>[2x]APTENSTGVQDCYRGDGQSYRGTLSTTITGRTCQSWSSMTPHWHRRIPLYYPN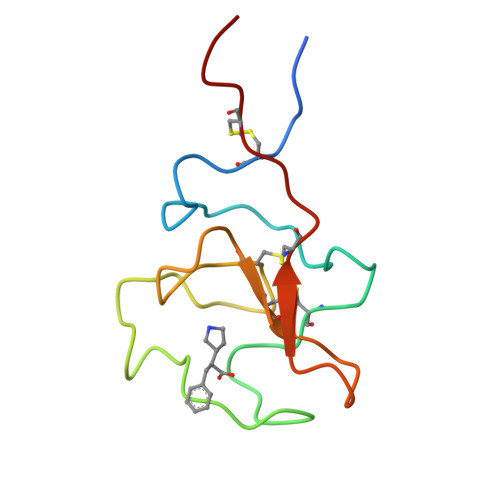AGLTRNYCRNPDAEIRPWCYTMDPSVRWEYCNLTRCPVTES>GGEVRQVSKHAFSLKQLDNPARIPPCGWKCSKCDMRENLWLNLTDGSILCGRRYFDGSGGNNHAVEH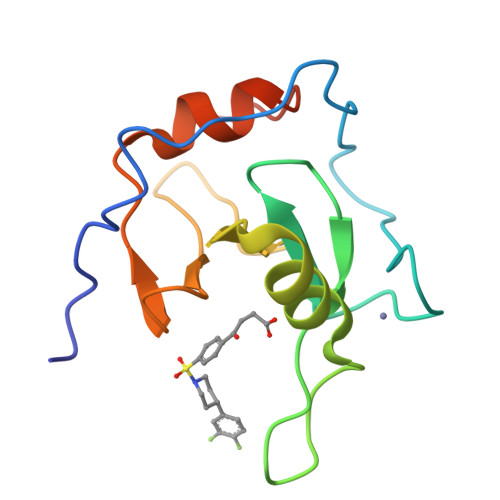YRETGYPLAVKLGTITPDGADVYSYDEDDMVLDPSLAEHLSHFGIDMLKMQKTD[2x]The rice NLR pair Pik-1/Pik-2 recognizes AVR-Pik effectors from the blast fungus Magnaporthe oryzae, triggering immune responses that limit rice blast infection. The sensor NLR Pik-1 harbours an integrated heavy metal associated (HMA) domain that directly binds AVR-Pik triggering immune responses. Allelic variation in a heavy metal associated (HMA) domain integrated in the receptor Pik-1 confers differential binding to AVR-Pik variants, determining resistance specificity. AVR-Pik is one of the several rice blast effectors characterized to date, and belongs to the Magnaporthe AVRs and ToxB like (MAX) effector family, whose members share a similar overall structural scaffold despite divergent sequence.

To gain a mechanistic understanding of how the Pikh Asn261Lys polymorphism increases the association of the receptor with AVR-Pik effectors, we determined the crystal structure of Pikh-HMA in complex with AVR-PikC. The complex was subsequently crystallised and X-ray diffraction data were collected at the Diamond Light Source (Oxford, UK) to 2.3 Å resolution. The position of Lys261 results in a different conformation for the C-terminal region of Pikh-HMA, compared to Pikp-HMA in complex with AVR-PikE. However, this conformation is similar to that observed in Pikm-HMA in complex with multiple AVR-Pik effectors. To date, there are no reported Pik NLR alleles that confer resistance to rice blast strains carrying AVR-PikC. This effector variant differs from AVR-PikE by a single polymorphism, Ala67Asp, located at the binding interface with the receptor. By contrast, in the structure of Pikh-HMA/AVR-PikC, the sidechain of Asp67 extends towards the HMA, and the nearby loop containing Asp224 is shifted away from the effector, likely as a consequence of steric clash and/or repulsion due to the matching charges of the two side chains. As a result, there are no hydrogen bonds formed between Asp224 of Pikh-HMA and Arg64 of AVR-PikC. Instead, the side chain of Arg64 forms an intramolecular hydrogen bond with the side chain of Asp67. We propose that disruption of hydrogen bonding network at this interface accounts for the lower binding affinity of Pik-HMA domains for AVR-PikC, and the lack of recognition of this effector by Pik NLR proteins in rice.

>GLKQKIVIKVAMEGNNCRSKAMALVASTGGVDSVALVGDLRDKIEVVGYGIDPIKLISALRKKVGDAELLQVSQAKKD[4x];>METGNKYIEKRAIDLSRERDPNFFDNPGIPVPECFWFMFKNNVRQDDGTCYSSWKMDMKVGPNWVHIKSDDNCNLSGDFPPGWIVLGKKRPGF[2x]> MGRDICTLDNVY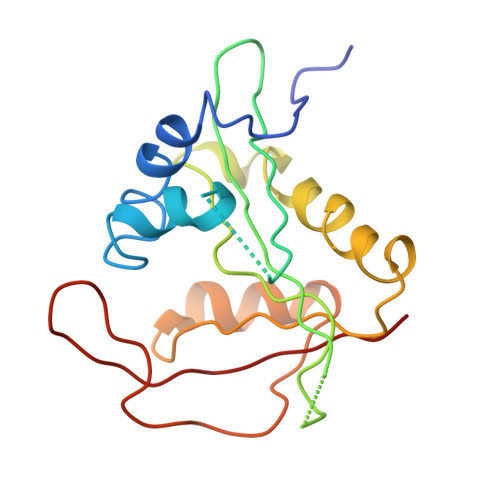ANNLGMLTKLAHVTVPNLYQDAFFSALFAEDSLVAKNKKPSSKKDVHFTQMAYYSEIPVGGLVAKLVPKKQNELSLKGIQIEFLGVLPNYRHKSIGSKLLKFAEDKCSECHQHNVFVYLPAVDDLTKQWFIAHGFEQVGETVNNFIKGVNGDEQDAILLKKHIS> MACNKQNGVKNILITFTHCDTGEVIGPISHEQPDDTLPTYKTCAWTNTALTNGAVMRSASNATMTLPVVRDPRVPLAWYQG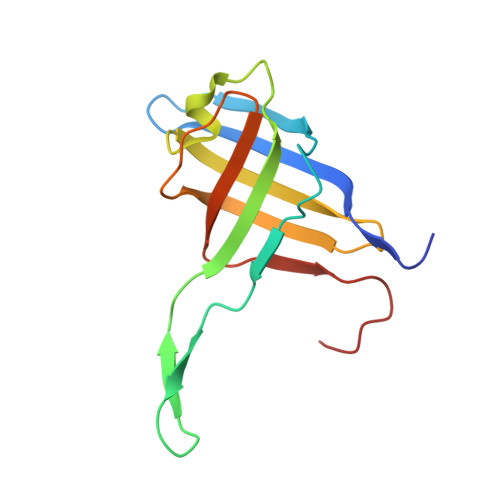CAQIDAQVEKFDGTVMTLTEGAVTEPEESDGRAVTMTIIAAEIDELLPPGSLAAA~{N}-(4-phenylazanylphenyl)ethanamide | C14 H14 N2 O | 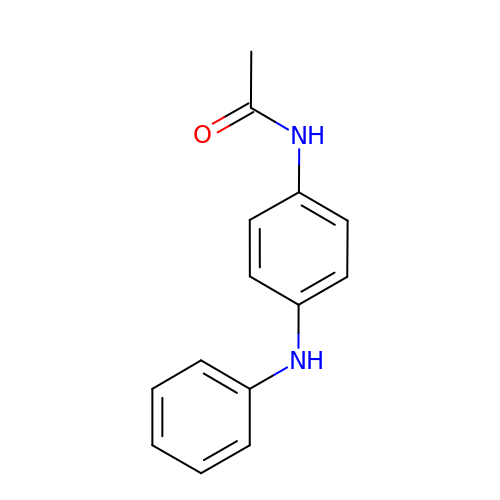QAIADKFUCPEVKW-UHFFFAOYSA-N Here we report a new antimicrobial peptide belonging to the cathelicidin family, cathelicidin-MH (cath-MH), from the skin of Microhyla heymonsivogt frog. Cath-MH has a single α-helical structure in membrane-mimetic environments and is antimicrobial against fungi and bacteria, especially Gram-negative bacteria. In contrast to other cathelicidins, cath-MH suppresses coagulation by affecting the enzymatic activities of tissue plasminogen activator, plasmin, β-tryptase, elastase, thrombin, and chymase. According to the amino acid sequences of known frog cathelicidins, the predicted mature cath-MH sequence (APCKLGCKIKKVKQKIKQKLKAKVNAVKTVIGKISEHLG) possessed 12 strongly basic residues distributed across the entire molecule, resulting in an 11 charge at pH 7.0.

The small trigonal-shaped crystals of the peptide were successfully grown under Crystal ScreenHT (Hampton Research) conditions of 2 M ammonium sulfate over 60 d at 277 K. While cath-MH crystals diffracted X-rays to 1.95 Å resolution, the crystal structure was solved at 2.20 Å resolution because the initial resolution did not provide a complete non-protein 2Fo - Fc electron density map. The peptide crystals belonged to the rhombohedral space group R32. The crystal asymmetric unit contained one molecule of the peptide with a solvent content of 41.76%. Loop-1 was formed by the first four amino acids A1-K4 at the N-terminal part of the structure, and loop-2 contained the last four amino acids E36-G39 at the C-terminal part. Non-protein electron density was interpreted as 13 water molecules and two chloride ions. The stabilization of the α-helical monomer was provided by a disulfide bridge formed from sulfur atoms of C3 and C7 and by several H-bonds between O atom C3 and Nζ atom K8 at 3.15 Å; between O atom Q25 and Oγ1 T29 at 2.70 Å; between O atom of I31 and Oγ S35 at 2.92 Å; and between Nζ K33 and Oε1 E36 at 2.68 Å distance. Further stabilization was realized by interactions between Sγ atom C3 with Nζ atom of K11; O atom of Q14 and Oε1 Q18; and Nζ atom of K17 and Nζ atom of K21. The monomer was more positively charged at the N-terminus than the C-terminus and shared high secondary structural similarity. Finally, compared to cathelicidin-PY, cath-MH contains a larger helix and five extra hydrogen bonds.

> APCKLGCKIKKVKQKIKQKLKAKVNAVKTVIGKISEHLG>[2x]CGCAA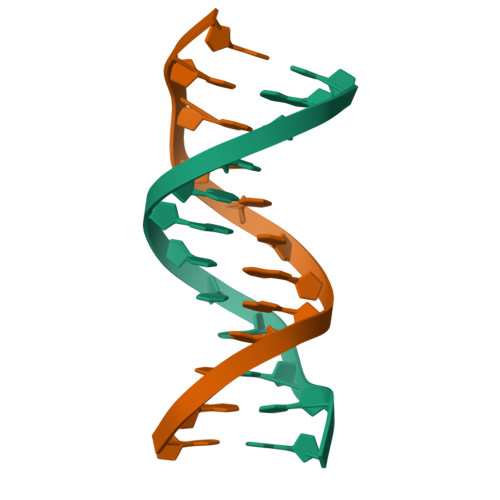ATTTGCG>MGKLLLILGSAIALPSFAAAGGDLDISDTVGVSFWLVTAGMLAATVFFFVERDQVSAKWKTSLTVS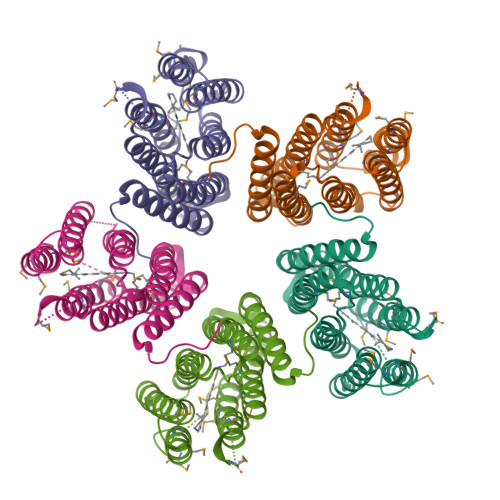GLITGIAFWHYLYMRGVWIDTGDTPTVFRYINWLLTVPLQVVEFYLILAACTSVAASLFKKLLAGSLVMLGAGFAGEAGLAPVLPAFIIGMAGWLYMIYELYMGEGKAAVSTASPAVNSAYNAMMMIIVVGWAIYPAGYAAGYLMGGEGVYASNLNLIYNLADFVNKILFGLIIWNVAVKESSNALEHHHHHH[5x]> GCUUCAACAACCCCGUAGGUGGGGACGAAAGUCAGCGCACCUACUG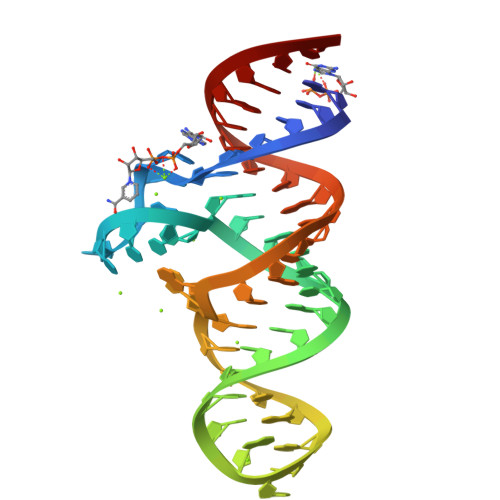GAGCC>[2x]MNRLPYFINYFFDTYLLISEDTPVGSSVTQLLARDLDNDPLVFGVVGEEASRFFAVESETGVVWLRQPLDRETKSEFT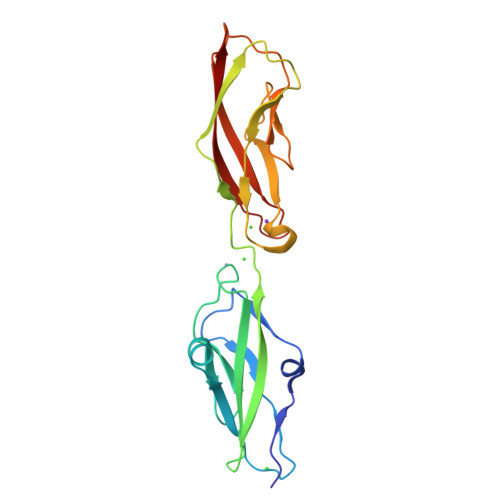VEFSVSDSQGVIKGTVNIQVGDVNDNAPRFHNQPYSVRIPENTPVGTPIFIVNATDPDQGAGGSVLYSFQPPSNFFAIDSGRGIVTVIRALDYEVTQAYQLQVNATDQDKTKPLSTLANLAITITD> MAHYPTRLKTRKTYSWVGRPLLDRKLHYQTYREMCVKTEGCSTEIHIQIGQFVLIEGDDDENPYVAKLLELFEDDSDPPPKKRARVQWFVRFCEVPACKRHLLGRKPGAQEIFWYDYPACDSNINAETIIGLVRVIPLAPKDVVPTNLKNEKTLFVKLSWNEKKFRPLSSELFAELNKPQESAAKCQKPVRAKSKSAESPSWTPAEHVAKRIESRHSASKSRQTPTHPLTPRARKRLELGNLGNPQMSQQTSCASLDSPGRIKRKVAFSEITSPSKRSQPDKLQTLSPALKAPEKTRETGLSYTEDDKKASPEHRIILRTRIAASKTIDIREERTLTPISGGQRSSVVPSVILKPENIKKRDAKEAKAQNEATSTPHRIRRKSSVLTMNRIRQQLRFLGNSKSDQEEKEILPAAEISDSSSDEEEASTPPLPRRAPRTVSRNLRSSLKSSLHTLTKVPKKSLKPRTPRCAAPQIRSRSLAAQEPASVLEEARLRLHVSAVPESLPCREQEFQDIYNFVESKLLDHTGGCMYISGVPGTGKTATVHEVIRCLQQAAQANDVPPFQYIEVNGMKLTEPHQVYVQILQKLTGQKATANHAAELLAKQFCTRGSPQETTVLLVDELDLLWTHKQDIMYNLFDWPTHKEARLVVLAIANTMDLPERIMMNRVSSRLGLTRMCFQPYTYSQLQQILRSRLKHLKAFEDDAIQLVARKVAALSGDARRCLDICRRATEICEFSQQKPDSPGLVTIAHSMEAVDEMFSSSYITAIKNSSVLEQSFLRAILAEFRRSGLEEATFQQIYSQHVALCRMEGLPYPTMSETMAVCSHLGSCRLLLVEPSRNDLLLRVRLNVSQDDVLYALKDE;> MSKPELKEDKMLEVHFVGDDDVLNHILDREGGAKLKKERAQLLVNPKKIIKKPEYDLEEDDQEVLKDQNYVEIMGRDVQESLKNGSATGGGNKVYSFQNRKHSEKMAKLASELAKTPQKSVSFSLKNDPEITINVPQSSKGHSASDKVQPKNNDKSEFLSTAPRSLRKRLIVPRSHSDSESEYSASNSEDDEGVAQEHEEDTNAVIFSQKIQAQNRVVSAPVGKETPSKRMKRDKTSDLVEEYFEAHSSSKVLTSDRTLQKLKRAKLDQQTLRNLLSKVSPSFSAELKQLNQQYEKLFHKWMLQLHLGFNIVLYGLGSKRDLLERFRTTMLQDSIHVVINGFFPGISVKSVLNSITEEVLDHMGTFRSILDQLDWIVNKFKEDSSLELFLLIHNLDSQMLRGEKSQQIIGQLSSLHNIYLIASIDHLNAPLMWDHAKQSLFNWLWYETTTYSPYTEETSYENSLLVKQSGSLPLSSLTHVLRSLTPNARGIFRLLIKYQLDNQDNPSYIGLSFQDFYQQCREAFLVNSDLTLRAQLTEFRDHKLIRTKKGTDGVEYLLIPVDNGTLTDFLEKEEEEA;> MATSSMSKGCFVFKPNSKKRKISLPIEDYFNKGKNEPEDSKLRFETYQLIWQQMKSENERLQEELNKNLFDNLIEFLQKSHSGFQKNSRDLGGQIKLREIPTAALVLGVNVTDHDLTFGSLTEALQNNVTPYVVSLQAKDCPDMKHFLQKLISQLMDCCVDIKSKEEESVHVTQRKTHYSMDSLSSWYMTVTQKTDPKMLSKKRTTSSQWQSPPVVVILKDMESFATKVLQDFIIISSQHLHEFPLILIFGIATSPIIIHRLLPHAVSSLLCIELFQSLSCKEHLTTVLDKLLLTTQFPFKINEKVLQVLTNIFLYHDFSVQNFIKGLQLSLLEHFYSQPLSVLCCNLPEAKRRINFLSNNQCENIRRLPSFRRYVEKQASEKQVALLTNERYLKEETQLLLENLHVYHMNYFLVLRCLHKFTSSLPKYPLGRQIRELYCTCLEKNIWDSEEYASVLQLLRMLAKDELMTILEKCFKVFKSYCENHLGSTAKRIEEFLAQFQSLDETKEEEDASGSQPKGLQKTDLYHLQKSLLEMKELRRSKKQTKFEVLRENVVNFIDCLVREYLLPPETQPLHEVVYFSAAHALREHLNAAPRIALHTALNNPYYYLKNEALKSEEGCIPNIAPDICIAYKLHLECSRLINLVDWSEAFATVVTAAEKMDANSATSEEMNEIIHARFIRAVSELELLGFIKPTKQKTDHVARLTWGGC;> MSSRKSKSNSLIHTECLSQVQRILRERFCRQSPHSNLFGVQVQYKHLSELLKRTALHGESNSVLIIGPRGSGKTMLINHALKELMEIEEVSENVLQVHLNGLLQINDKIALKEITRQLNLENVVGDKVFGSFAENLSFLLEALKKGDRTSSCPVIFILDEFDLFAHHKNQTLLYNLFDISQSAQTPIAVIGLTCRLDILELLEKRVKSRFSHRQIHLMNSFGFPQYVKIFKEQLSLPAEFPDKVFAEKWNENVQYLSEDRSVQEVLQKHFNISKNLRSLHMLLMLALNRVTASHPFMTAVDLMEASQLCSMDSKANIVHGLSVLEICLIIAMKHLNDIYEEEPFNFQMVYNEFQKFVQR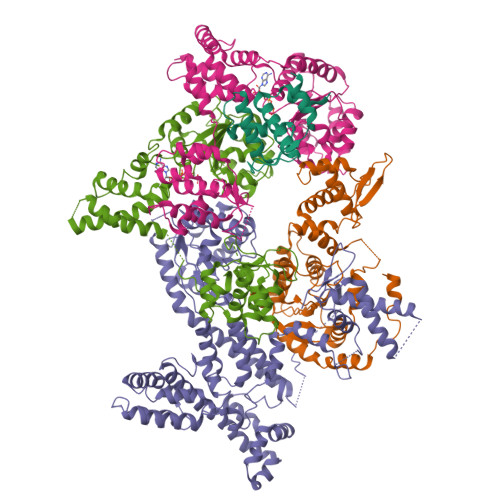KAHSVYNFEKPVVMKAFEHLQQLELIKPMERTSGNSQREYQLMKLLLDNTQIMNALQKYPNCPTDVRQWATSSLSWL;> MPHLENVVLCRESQVSILQSLFGERHHFSFPSIFIYGHTASGKTYVTQTLLKTLELPHVFVNCVECFTLRLLLEQILNKLNHLSSSEDGCSTEITCETFNDFVRLFKQVTTAENLKDQTVYIVLDKAEYLRDMEANLLPGFLRLQELADRNVTVLFLSEIVWEKFRPNTGCFEPFVLYFPDYSIGNLQKILSHDHPPEYSADFYAAYINILLGVFYTVCRDLKELRHLAVLNFPKYCEPVVKGEASERDTRKLWRNIEPHLKKAMQTVYLREISSSQWEKLQKDDTDPGQLKGLSAHTHVELPYYSKFILIAAYLASYNPARTDKRFFLKHHGKIKKTNFLKKHEKTSNHLLGPKPFPLDRLLAILYSIVDSRVAPTANIFSQITSLVTLQLLTLVGHDDQLDGPKYKCTVSLDFIRAIARTVNFDIIKYLYDFL methyl 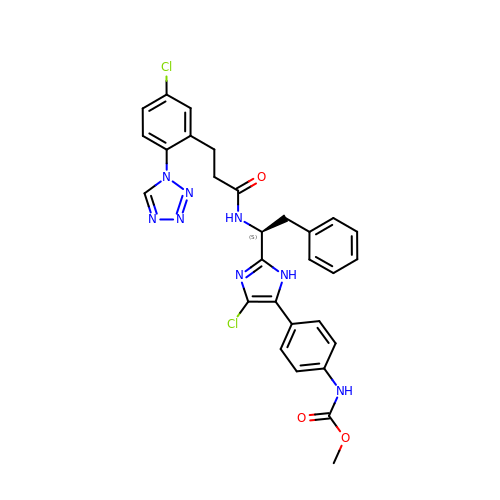(4-{4-chloro-2-[(1S)-1-({3-[5-chloro-2-(1H-tetrazol-1-yl)phenyl]propanoyl}amino)-2-phenylethyl]-1H-imidazol-5-yl}phenyl)carbamate | C29 H26 Cl2 N8 O3 | QPRIEKZFCOMXST-QHCPKHFHSA-N>MRGSHHHHHHGSTSSSTPRHRGIFPVVPTTFADTGELDLASQKRAVDFMIDAGSDGLCILANFSEQFAITDDERDVLTRTILEHVAGRVPVIVTTSHYSTQVCAARSLRAQQLGAAMVMAMPPYHGATFRVPEAQIFEFYARVSDAIAIPIMVQDAPASGTALSAPFLARMAREIEQVAYFKIETPGAANKLREL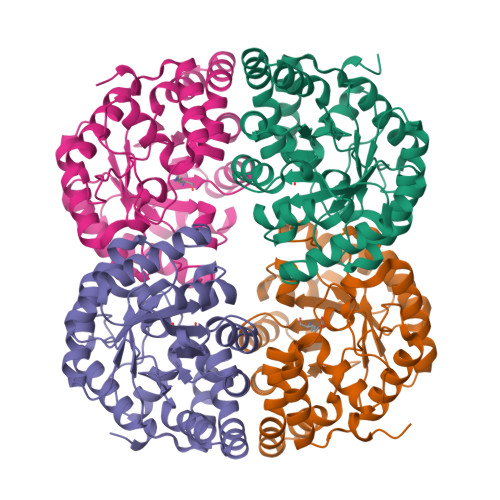IRLGGDAIEGPWDGEEAITLLADLHAGATGAMTGGGFPDGIRPILEAWREGRHDDAYARYQAWLPLINHENRQSGILTAKALMREGGVIASERPRHPMPELHPDTRAELLAIARRLDPLVLRWAH[12x]2-[3,6-bis(oxidanylidene)-4,5-dihydroxanthen-9-yl]-4-[3-[(2R)-2-oxidanylpropoxy]propylcarbamoyl]benzoic acid | C27 H27 N O8 | 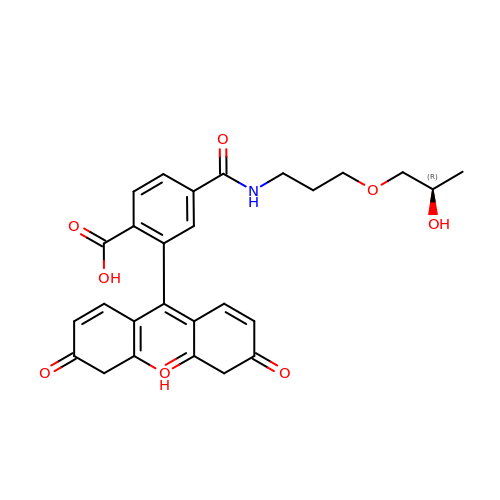GVYCNBHUBWDBFF-OAHLLOKOSA-N> MSLNVIDLFSGVGGLSLGAARAGFDVKMAVEIDQHAINTHAINFPRSLHVQEDVSLLNAEIIKGFFKNDMPIDGIIGGPPCQGFSSIGKGNPDDSRNQLYMHFYRLVSELQPLFFLAENVPGIMQEKYSGIRNKAFNLVSGDYDILDPIKVKASDYGAPTIRTRYFFIGVKKSLKLDISDEVFMPKMIDPVTVKDALYGLPDIIDANWQSDSESWRTIKKDRKGGFYEKLWGQIPRNVGDTESIAKLKNNIISGC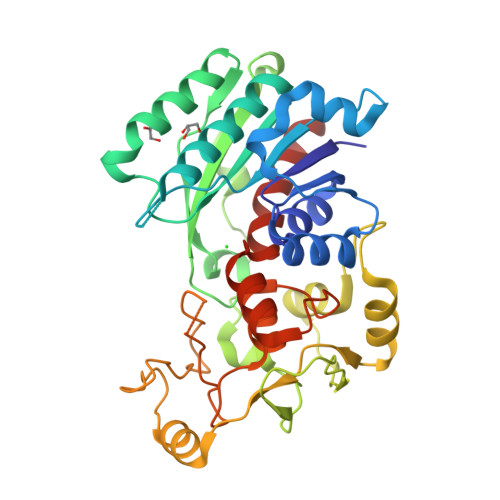TGTLHSKIVQERYASLSFGETDKISRSTRLDPNGFCPTLRAGTARDKGSFQAVRPIHPYHPRVITPREAARLQGFPDWFRFHVTKWHSFRQIGNSVSPIVAEYILKGLYNLLNEGHHHHHH>[6x]MATKGTKRSYEQMETDGERQNATEIRASVGKMIDGIGRFYIQMCTELKLSDYEGRLIQNSLTIERMVLSAFDERRNKYLEEHPSAGKDPKKTGGPIYRRVDGKWRRELILYDKEEIRRIWRQANNGDDATAGLTHMMIWHSNLNDATYQRTRALVRTGMDPRMCSLMQGSTLPRRSGAAGAAVKGVGTMVMELIRMIKRGINDRNFWRGENGRRTRIAYERMCNILKGKFQTAAQRTMVDQVRESRNPGNAEFEDLIFLARSALILRGSVAHKSCLPACVYGSAVASGYDFEREGYSLVGIDPFRLLQNSQVYSLIRPNENPAHKSQLVWMACHSAAFEDLRVSSFIRGTKVVPRGKLSTRGVQIASNENMETMESSTLELRSRYWAIRTRSGGNTNQQRASSGQISIQPTFSVQRNLPFDRPTIMAAFTGNTEGRTSDMRTEIIRLMESARPEDVSFQGRGVFELSDEKATSPIVPSFDMSNEGSYFFGDNAEEYDN

In total, the genome of influenza A virus encodes eleven proteins, i.e. haemagglutinin (HA), neuraminidase (NA), nucleoprotein (NP), matrix protein (M1 and M2), non-structure proteins (NS1 and NS2) and polymerase (PA, PB1, PB1- F2 and PB2). Among them, NP is regarded as an attractive target due to its highly conservative and multifunctional nature during virus life cycle. Interestingly, Kao et al. identified NP as an anti-influenza drug target using advanced chemical genetics approach, and reported that a novel small molecule named nucleozin could target this protein. NP forms large aggregates in the presence of nucleozin, and is restrained from nuclear accumulation, which in turn results in cessation of virus replication.

The crystal structure of nucleozin bound H1N1 NP has been solved at a resolution of 3.0 Å and there are six NP molecules assembled into two trimers in the crystallographic asymmetric unit. In the current structure, two nucleozin compounds were found to bridge the two trimers in the asymmetric unit forming a dimer of trimers. There are six NP molecules in the asymmetric unit while only two nucleozin molecules were identified in the structure. It is very clear that one nucleozin molecule bridges two NP molecules in two adjacent trimers, and the binding pockets are formed by combination of the Y289/N309 pocket from one NP molecule and R382 pocket from the other NP molecule. The Y289/N309 pocket is composed of hydrophobic interactions with side chains of residues Y289, F291, L306, R305 and N309. In this pocket, the aromatic ring of residue Y289 forms hydrophobic interactions with the phenyl ring part of nucleozin through π stacking. Residue N309 forms both hydrophobic and weak hydrogen bond interactions with the middle part of nucleozin. The R382 pocket, composed of residues R382 and R384, supports the nitro-phenyl moiety of nucleozin like a horse saddle. In the NP-nucleozin complex structure, nucleozin molecules only bind with Y289/N309 pockets from Chain A and Chain D, and it has not been found in the other four Y289/N309 pockets and none of the Y52/Y313 pockets as revealed in the nucleozin analog-NP structure. The underlying reasons might be that, the interaction between nucleozin and Y289/N309 pocket is essential but not enough for their binding, so only these two Y289/N309 pockets in Chain A and D which get additional support from the R382 pocket in an adjacent NP chain are able to stabilize nucleozin molecules. Based on the structure, we propose that nucleozin could link two NP molecules into dimeric subunits, and then further induce the formation of large aggregates, which is illustrated in our computational models.> SYAFFVQTCREEHKKKHPDASVNFSEFSKKCSERWKTMSAKEKGKFEDMAKADKARYEREMKTYIPPKGETK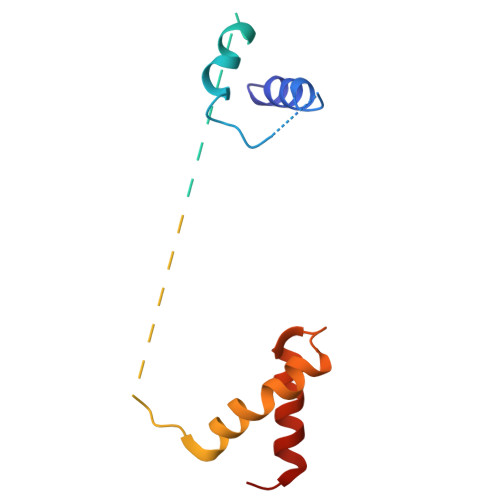KKFKDPNAPKRPPSAFFLFCSEYRPKIKGEHPGLSIGDVAKKLGEMWNNTAADD> TFEYGDGI;> MAIYADNSYSIGNTPLVRLKHFGHNGNVVVKIEGRNPSYSVKCRIGANMVWQAEKDGTLTKGKEIVDATSGNTGIALAYVAAARGYKITLTMPETMSLERKRLLCGLGVNLVLTEGAKGMKGAIAKAEEIVASDPSRYVMLKQFENPANPQIHRETTGPEIWKDTDGKVDVVVAGVGTGGSITGISRAIKLDFGKQITSVAVEPVESPVISQTLAGEEVKPGPHKIQGIGAGFIPKNLDLSIIDRVETVDSDTALATARRLMAEEGILAGISSGAAVAAA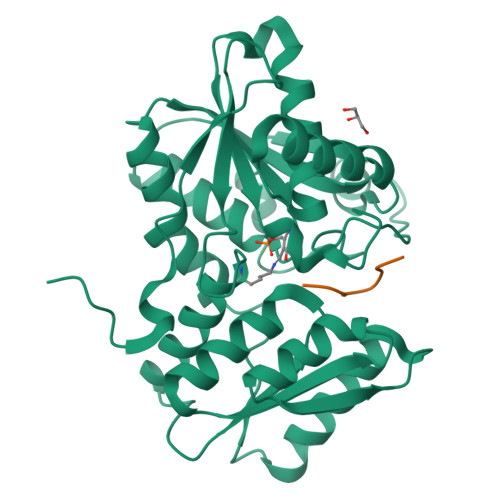DRLAKLPEFADKLIVVILPSASERYLSTALFEGIEG>[4x]MSLGALPTAEDIDAVVLDFDGTQTDDRVLIDSDGREFVSVHRGDGLGIAALRKSGLTMLILSTEQNPVVAARARKLKIPVLHGIDRKDLALKQWCEEQGIA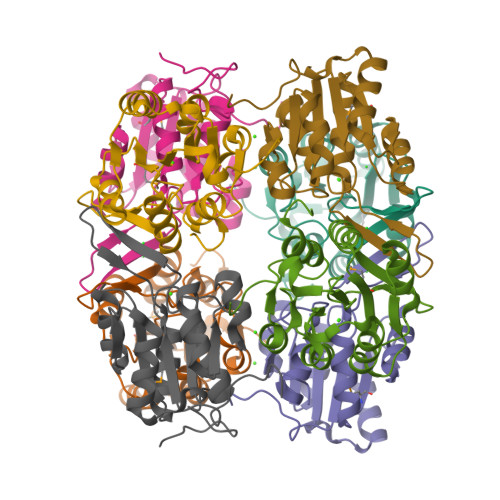PERVLYVGNDVNDLPCFALVGWPVAVASAHDVVRGAARAVTTVPGGDGAIREIASWILGPSLDSLDKEGHHHHHH>[6x]MGSDKIHHHHHHMEYKKFVEARRELNEKVLSRGTLNTKRFFNLDSAVYRPGKLDVKTKELMGLVASTVLRCDDCIRYHLVRCVQEGASDEEIFEALDIALVV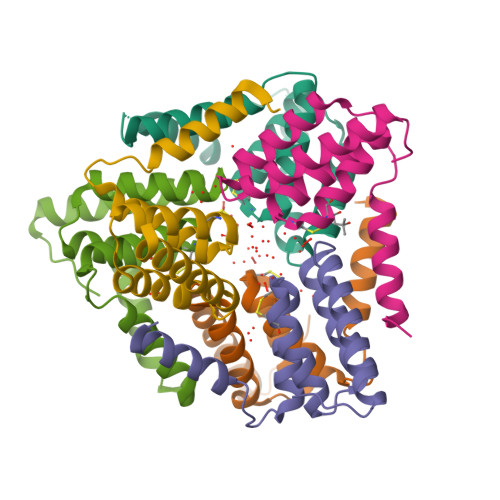GGSIVIPHLRRAVGFLEELREMEKNGETISL>MEKRMSTQQRAAGNACPTAAFSFDPARLAQRRRWAGAFAALCGLALSPSALLAEEHSQHQDHAVELAPSVVTGVAQ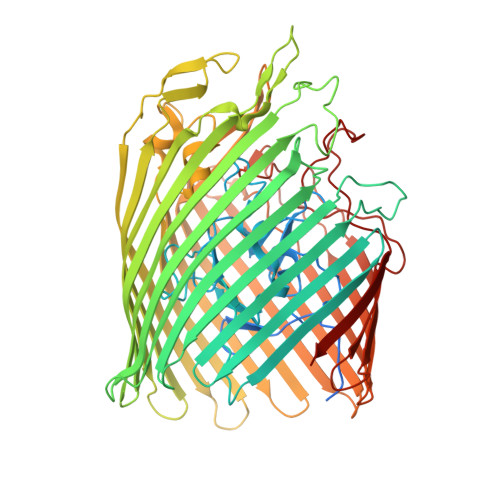SSPLTIVTNPKEPRQPVPASDGADYLKTIPGFAVIRNGGSNGDPVLRGMFGSRLNILTNGGMMLGAAPNRMDAPTSYISPETYDKLTVIKGPQTVLWGPGASAGTILFEREPERFGELGSRVNASLLAGSNGRFDKVLDAAAGNRLGYLRFTGNHAQSDDYEDGAGNTVPSRWKKWNGDVAVGWTPDEDTLIELTAGKGDGEARYAGRGMDGSQFKRESLGLRFVKSNVSDVLEKVEAQVYYNYADHIMDNFRLRTPDPSSMMPMPMASQVDRRTLGGRLAATWRWDDFKLVTGVDAMRNEHRARGSKYDMMTDYYTDADQFPWSKDAVFHNYGAFGELTWFAAERDRLIGGLRLDRASVKDYRQTLKSGHMGHAMANPTANDTRADTLPSGFVRYEHDLADSPTTLYAGLGHAERFPDYWELFSPKRGPNGSVNAFDKIKPEKTTQLDFGLQYNGDKLQAWASGYVGVVQDFILFSYREGMMGSSTQATNVDARIMGGELGASYQLTGNWKTDASLAYAWGKNSSDDRALPQIPPLEARFGLTYEEGDWSAGSLWRVVAPQNRIARDQGNVVGKDFDKSAGFGVFSLNGAYRVTRNVKLSAGVDNLFDKDYTEHLNKAGDAGFGFSANETVPEPGRTFWTKVDFSF[2x]>[2x]GSHMSMYNMDLDKVIRKINKKGARTVGLQFPEGLKMQAVKIAKAIESQTPATVIISGDPCFGACDVSDYKMKGSVDLIVHYGHTPLPLKYEVPTLFIEAFSNIDVKKDLEKCLEKLEDYSKIALVTT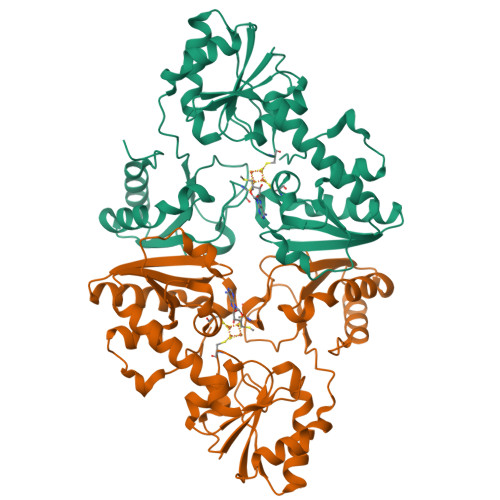TQHLHLLNEIKDYLEDNGKEVVLGSSKNTKKGQVLGCNFSSIKNLDAEVYLFIGSGNFHPLGIYLFTKSPVLALDPYNSEIRDISAFADRILRIRFARITKAREAEKWGIIVSSKEGQYRMKLAKEIKKILEDNKMEAYIIMADNINPDILLPYMELDAFVVSACPRIAIDDSQMYKKPLLTPQELEIVLNKRQWENYQLDEILFHERYK1-(4-carbamimidamidobutyl)guanidine | C6 H16 N6 | 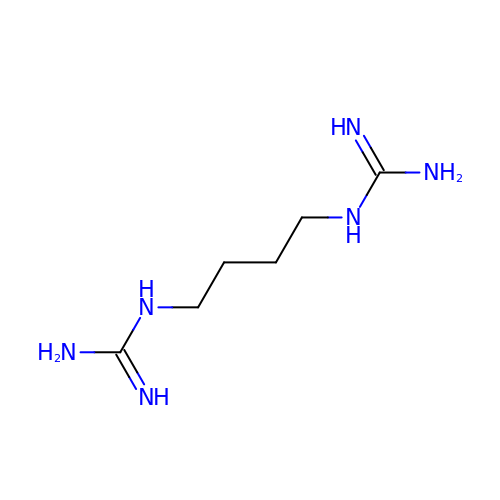HGMDNMBBCKDWTQ-UHFFFAOYSA-N>GPCTSFPQALCVQWKNAYALCWLDCILSALVHSEELKNTVTGLCSKEESIFWRLLTKYNQANTLLYTSQLSGVKDGDCKKLTSEIFAEIETCLNEVRDEIFISLQPQLRCTLGDMESPVFAFPLLLKLETHIEKLFLYSFSWDFECSQCGHQYQNRHMKSLVTFTNVIPEWHPLNAAHFGPCNNCNSKSQIRKMVLEKVSPIFMLHFVEGLPQNDLQHYAFHFEGCLYQITSVIQYRANNHFITWILDADGSWLECDDLKGPCSERHKKFEVPASEIHIVIWERKIS[2x];>[2x]SEEKPKEGVKTENDHINLKVAGQDGSVVQFKIKRHTPLSKLMKAYCERQGLSMRQIRFRFDGQPINETDTPAQLEMEDEDTIDVFQQQTG

Ub/Ubl protein conjugation can be reversed by specialized isopeptidases termed deubiquitinases (DUBs) or Ubl proteases, which antagonize Ub/Ubl-mediated post-translational modifications. Moreover, we focused on recently structurally characterized USPL1, which is the only deSUMOylase with a USP fold but for which its mechanism for SUMO paralogue specificity had remained unclear. USPL1 featured an approximately 25-fold higher activity for SUMO2 over SUMO1, which suggests a much more pronounced paralogue specificity as previously assumed from fluorogenic reagents. We structurally and biochemically explain this substrate selection, as USPL1 uses the USP fingers subdomain to contact the Gly27/Gly26 loop of SUMO2/3 to discriminate against SUMO1.

Taking inspiration from Ubiquitin- and ISG15-processing USP-substrate complexes, we semisynthetically obtained SUMO activity-based probes that contain a reactive warhead at the protein’s C-terminus. SUMO2 and SUMO3 feature identical Ubl folds and differ only in their unstructured N-terminal extensions. We prepared a SUMO3–2Br probe with a 2-bromoethyl warhead as well as a ΔN-SUMO2/3-PA probe equipped with a propargylamine warhead. Both probes reacted covalently with USPL1 as evident from a shift in molecular weight and led to pronounced protein stabilization as assessed by protein melting temperature analysis, indicative of the specific recognition of SUMO by USPL1. We solved crystal structures of USPL1 in covalent complex with ΔN-SUMO2/3-PA to 2.4 Å resolution, as well as of USPL1 in complex with SUMO3–2Br to 2.17 Å resolution in a different crystal form. The latter structure featured two almost identical copies in the asymmetric unit and was used for single-wavelength anomalous dispersion measurements with a selenomethionine-containing SUMO3–2Br probe. Alignment of the catalytic triad Cys236, His456, and Asp472 in the SUMO3–2Br probe-bound structure was observed, and the importance of the respective residues for enzymatic activity as well as probe reactivity was confirmed by mutation. Alignment of three independently obtained relative arrangements of the USPL1 and SUMO folds revealed near-identical positioning of SUMO in these highly conserved areas including the SUMO C-terminus, the Pro66 loop, as well as the Gly27 loop in the fingers. Strikingly, mutation of Gly27 into serine abolished USPL1 activity completely, in line with Gly27’s central structural role in anchoring of the SUMO fold into the USPL1 fingers.> DFNNLTKGLCTINSWHIYGKDNAVRIGEDSDVLVTREPYVSCDPDECRFYALSQGTTIRGKHSNGTIHDRSQYRALISWPLSSPPTVYNSRVECIGWSSTSCHDGKT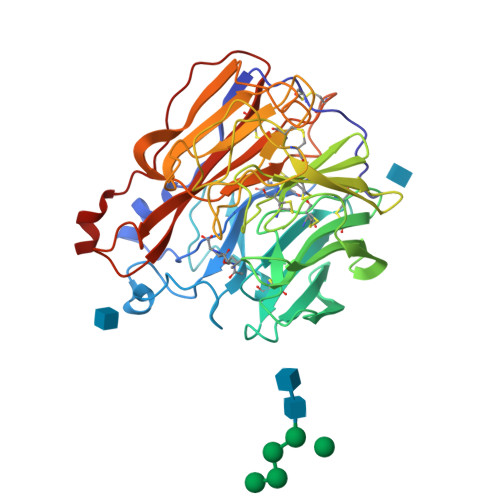RMSICISGPNNNASAVIWYNRRPVTEINTWARNILRTQESECVCHNGVCPVVFTDGSATGPAETRIYYFKEGKILKWEPLAGTAKHIEECSCYGERAEITCTCRDNWQGSNRPVIRIDPVAMTHTSQYICSPVLTDNPRPNDPTVGKCNDPYPGNNNNGVKGFSYLDGVNTWLGRTISIASRSGYEMLKVPNALTDDKSKPTQGQTIVLNTDWSGYSGSFMDYWAEGECYRACFYVELIRGRPKEDKVWWTSNSIVSMCSSTEFLGQWDWPDGAKIEYFL> HMSPGDSRRLSIQRCIQSLVHACQCRNANCSLPSCQKMKRVVQHTKGCKRKTNGGCPICKQLIALCCYH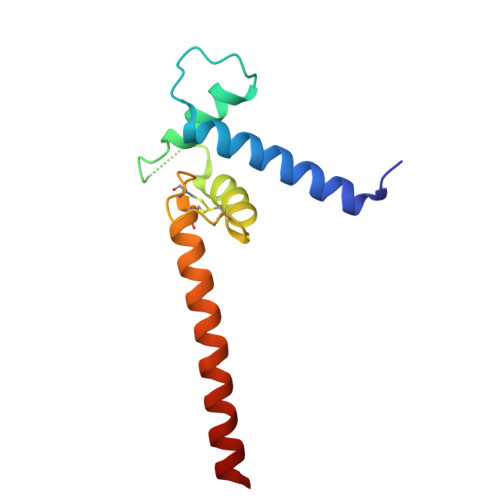AKHCQENKCPVPFCLNIKQKLRQQQLQHRLQQAQMLRRRMASM>MSTVHEILCKLSLEGDHSTPPSAYGSVKPYTNFDAERDALNIETAVKTKGVDEVTIVNILTNRSNVQRQDIAFAYQRRTKKELPSALKSALSGHLETVILGLLKTPAQYDASELKASMKGLGTDEDSLIEIICSRTNQELQEINRVYKEMYKTDLEKDIISDTSGDFRKLMVALAKGRRAEDGSVIDYELIDQDARELYDAGVKRKGTDVPKWISIMTERSVCHLQKVFERYKSYSPYDMLESIKKEVKGDLENAFLNLVQCI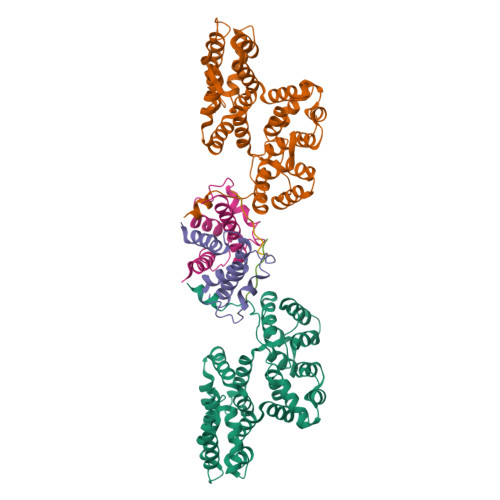QNKPLYFADRLYDSMKGKGTRDKVLIRIMVSRSEVDMLKIRSEFKRKYGKSLYYYIQQDTKGDYQKALLYLCGGDD[4x];>[4x]SPSQMEHAMETMMFTFHKFAGDKGYLTKEDLRVLMEKEFPGFLENQKDPLAVDKIMKDLDQCRDGKVGFQSFFSLIAGLTIACNDYFVVHMKQKGKK;>[4x]PRLSYPTFFPRFEF> GPYYPTNKLQAAVMETDRENAIIRQRNDEIPTRTLDTAIFTD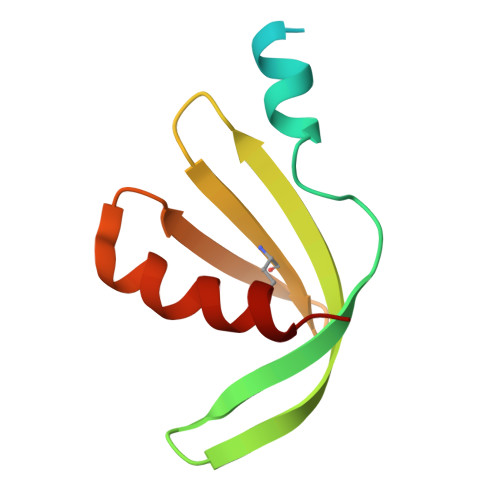ASTVASAQIHLYYNSNIGKIIMSLNGKKHTFNLYDDNDIRTLLPILLLSK>[4x]MGSSHHHHHHSSGLVPRGSHMASYALNNNSDFNNGWKFTLSDSVCYSFVNYNPSSWKTVNLPHDWSVDLPFESTAEGCTGFLKGGIGWYSKTFDTPDNFVDKKCYIVFDGVYNNSEYWINGRKLGFHPYGYSPFFYDISDYLNPKGQENRISVRIDHSRYADSRWYTGSGIYRETQLIFTDKLHIPVWGTFVTTPVVSSERATVNIEVRVKNDYSGPRAGEVRTSYFDSKNKKVGEKLTSFLIEAGKEMKINQSVEISNPSLWDVDSPSMYLAKSEILVDGNVVDTKETPFGIRSIKFDAKKGFFLNGKNMKIKGVCLHHDASMIGAALVEDVWRRRLQTLKDGGCNAIRLSHNPGADAFLELCDEMGFLVQEEFFDEWDYPKDKRLNMDEQSIDYITRGYCEYFQEWAERDLKNVMLRSRNHPCIFQWSIGNEIEWTYKGCKESTGFFSADAGGGYFWNQPPYSTQRIREEWAKQPKQTYDIGRTAKKLAAWTREMDTTRPVTANCILPSISYETGYIDALDVAGFSYRRVMYDYAHKNYPDKPAMGTENLGQWHEWKAVIERDYIPGMFIWTGVDYLGEVGTKGREWPQRAIGCGLLDLAGFEKPSFHMMKSLWTDAPFIAIYSQTANKSSYVEKDGKFTDKDPKKPWTQRLWVWEDVNSHWNYTKGEKVVVEIYSNCDEIELFQNGKSLGKRFLKDFEDHIYKWSVDFKDGNIVAKGKKNGKKTTSAIYTTKETNSIKLSVDKVAVDANNTDVIHVTAQLIDRNGRNISWEEKEITFNIGGNYRLLGVENGDHLNVLNYKSNTVKTYKGRALLVLQATDKAGILNINANSGSISSNDLKVEVK

determined the three-dimensional structures of these four agarases. initiated by GH86 or GH16B, which generates NAOS. depolymerized by GH86, and systematically saccharified by the exo-acting GH117B and GH2C enzymes. exo-acting β-d-galactosidases, while GH117A and GH117B are α-1,3-L-neoagarooligosaccharide hydrolases.

replaced with W657 and C598 in GH2C, respectively. to specifically accommodate the β-linked AHG residue. generate AOS products, which are substrates for GH2C. AOS by GH117B and GH2C, respectively.> GLVPRGSHMRIALMQHTARPLDPQHNLDLIDDAAARASEQGAQLLLTPELFGFGYVPSQICAQVSAEQVDAARSRLRGIARDRGIALVWSLPGPEGPEQRGITAELADEHGEVLASYQKVQLYGPEEKA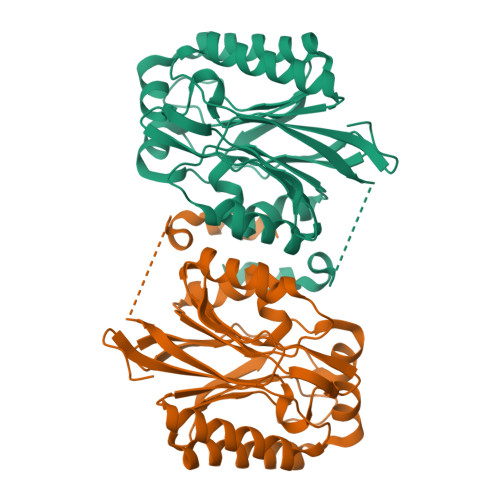AFVPGEQPPPVLSWGGRQLSLLVAYDVEFPEMVRAAAARGAQLVLVPTALAGDETSVPGILLPARAVENGITLAYANHCGPEGGLVFDGGSVVVGPAGQPLGELGVEPGLLVVDLPDQSQDAGSDSADYLQDRRAELHRNWL>GPLGSEEDVPENNGILISIKEVINAEFSRDGTIHSSELKGVLELRINDHDLSHSNLKLADSIDVRDKSFQFKTHPNIDKQSFLSTKLISLRDKSKAFPANDQSLGVLRWRKVAPAEDDSLIPLTLTTAVSPSESQQGFDVIIEYESVLETELADVIFTIPVFPQEPVDINTESSTCSDAEVVNMDQEMGTSIKISKIAANDAGALAFTIEAPYEDALYPMTVSFQESTRD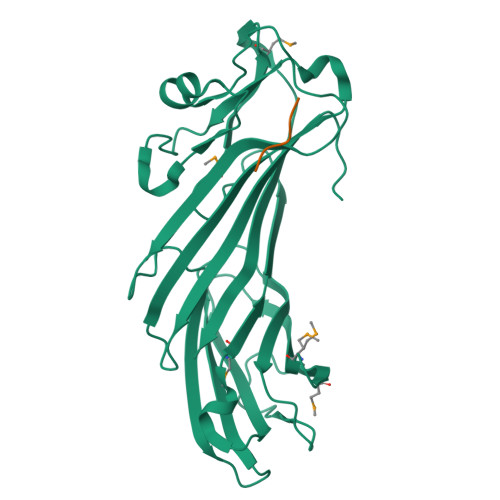KLAKSFTGMAIQSVVMANDHDQELPYDVITSLKSDEYLVQ[3x];>DEDKWDDF[2x]> MSTKTNSTKATSEKTDSLKTNSGTKSSAGYSEQNTPLGGCILADTPITFNENKPVTKVKVRNTGDRPIQVGSHFHFFEVNRALE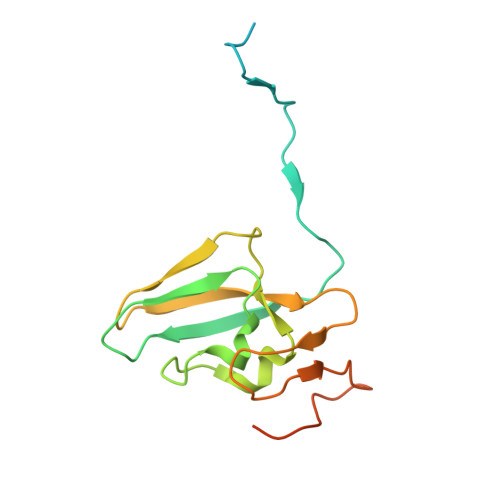FDRAAAYGKRLNISSTTAIRFEPGDETEVPLIPFGGKQTLYGFNNLVDGWTGEGVVPNSERPDKLEAIRRAAERGFKSSK>MGQGNDTSEVMLLDTGWEFSQSGTEKWMPATVPGTVHQDLISHELLPNPFYGMNEKKIQWVENEDWEYRTSFIVSEEQLNRDGIQLIFEGLDTYADVYLNGSLLLKADNMFVGYTLPVKSVLRKGENHLYIYFHSPIRQTLPQYASNGFNYPADNDHHEKHLSVFSRKAPYSYGWDWGIRMVTSGVWRPVTLRFYDIATISDYYVRQLSLTDENARLSNELIVNQIVPQKIPAEVRVNVSLNGTTVTEVKQQVTLQPGINHITLPAEVTNPVRWMPNGWGTPTLYDFSAQIACGDRIVAEQSHRIGLRTIRVVNEKDKDGESFYFEVNGIPMFAKGANYIPQDALLPNVTTERYQTLFRDMKEANMNMVRIWGGGTYENNLFYDLADENGILVWQDFMFACTPYPSDPTFLKRVEAEAVYNIRRLRNHASLAMWCGNNEILEALKYWGFEKKFTPEVYQGLMHGYDKLFRELLPSTVKEFDSDRFYVHSSPYLANWGRPESWGTGDSHNWGVWYGKKPFESLDTDLPR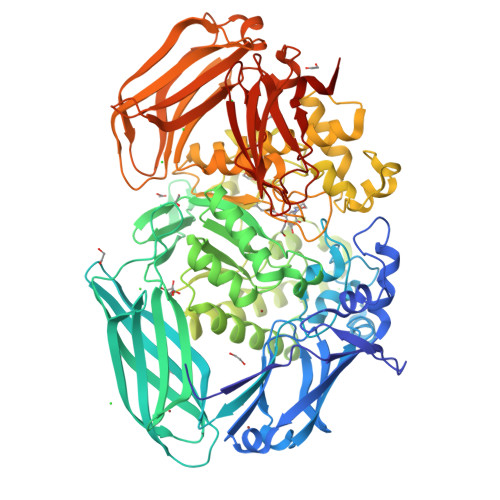FMSEFGFQSFPEMKTIAAFAAPEDYQIESEVMNAHQKSSIGNSLIRTYMERDYIIPESFEDFVYVGLVLQGQGMRHGLEAHRRNRPYCMGTLYWQLNDSWPVVSWSSIDYYGNWKALHYQAKRAFAPVLINPIQQNDSLSVYLISDRLDTMEQMTLEMKVVDFDGKTLGKKIQVHSLEVPANTSKCVYRAKLDGWLTPEDCRRSFLKLILKDKSGHQVAESVHFFRKTKDLQLPPTSVSYQMKQTDGKCELTLFSSMLAKDIFIETPLQGARYSDNFFDLLPGERKKVIITSPRIKKGEELPVNIKHIRETYKLEHHHHHH[2x]>[2x]AK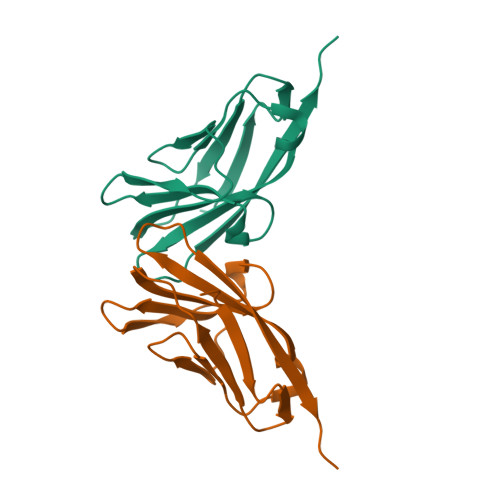LTIESTPFNVAEGKEVLLLVHNLPQHLFGYSWYKGERCDGNRQIIGYVIGTQQATPGPAYSGREIIYPNASLLIQNIIQNDAGFYTLHVIKSDLVNEEATGQFRVYPEL> GSMSLRPSERVEVRRNRYKVAVDAEEGRRRREDNMVEIRKSRREESLLKKRREGLQAQAPVPASAATGVDKKLESLPAMIGGVYSDDNNLQL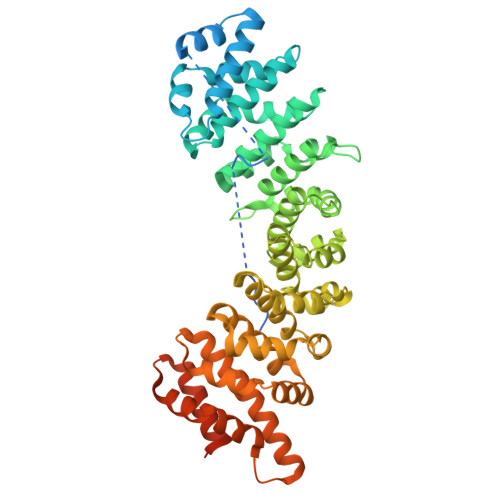EATTQFRKLLSIERSPPIEEVIQSGVVPRFVQFLTREDFPQLQFEAAWALTNIASGTSENTKVVIDHGAVPIFVKLLGSSSDDVREQAVWALGNVAGDSPKCRDLVLANGALLPLLAQLNEHTKLSMLRNATWTLSNFCRGKPQPSFEQTRPALPALARLIHSNDEEVLTDACWALSYLSDGTNDKIQAVIEAGVCPRLVELLLHPSPSVLIPALRTVGNIVTGDDAQTQCIIDHQALPCLLSLLTQNLKKSIKKEACWTISNITAGNKDQIQAVINAGIIGPLVNLLQTAEFDIKKEAAWAISNATSGGSHDQIKYLVSEGCIKPLCDLLICPDIRIVTVCLEGLENILKVGETDKTLAAGDVNVFSQMIDEAEGLEKIENLQSHDNNEIYEKAVKILEAYWMDEEDDTMGATTVAAPQGATFDFGQGGGAAQFK3-(2-fluorophenyl)benzoic acid | C13 H9 F O2 | 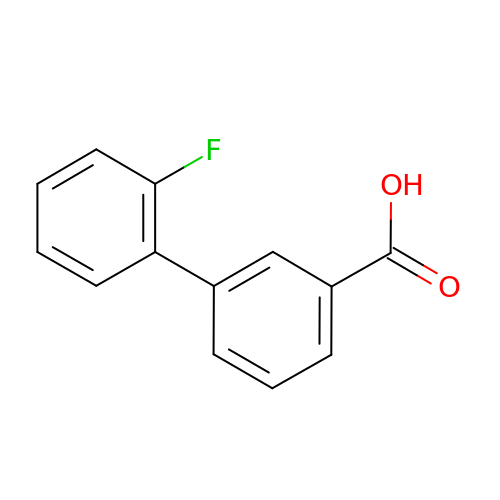KJRAPRROUUCCPO-UHFFFAOYSA-N4H,5H-naphtho[1,2-b]thiophene-2-carboxylic 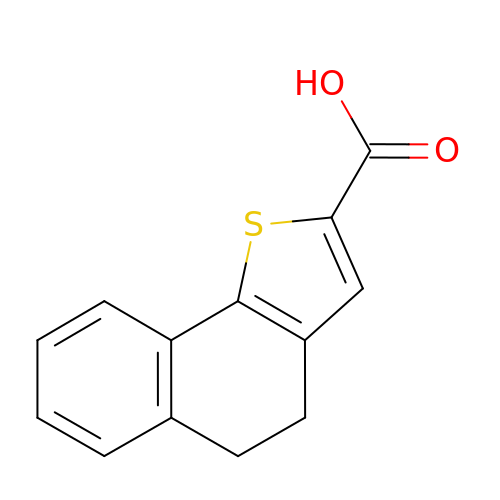acid | C13 H10 O2 S | IGBRCZHGFVMFCR-UHFFFAOYSA-N> MDEFEMIKRNTSEIISEEELREVLKKDEKSAYIGFE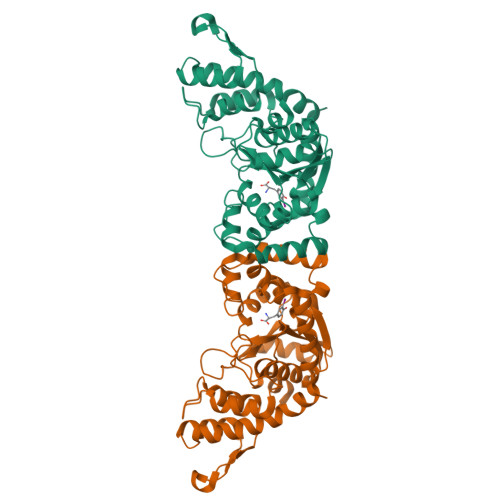PSGKIHLGHYLQIKKMIDLQNAGFDIIILLADLAAYLNQKGELDEIRKIGDYNKKVFEAMGLKAKYVYGSEFQLDKDYTLNVYRLALKTTLKRARRSMELIAREDENPKVAEVIYPIMQVNTSHYLGVDVAVGGMEQRKIHMLARELLPKKVVCIHNPVLTGLDGEGKMSSSKGNFIAVDDSPEEIRAKIKKAYCPAGVVEGNPIMEIAKYFLEYPLTIKRPEKFGGDLTVNSYEELESLFKNKELHPMYLKNAVAEELIKILEPIRKRLLEHHHHHH> GKDNFDAPESKLVGRVTYQGQALNLRGTG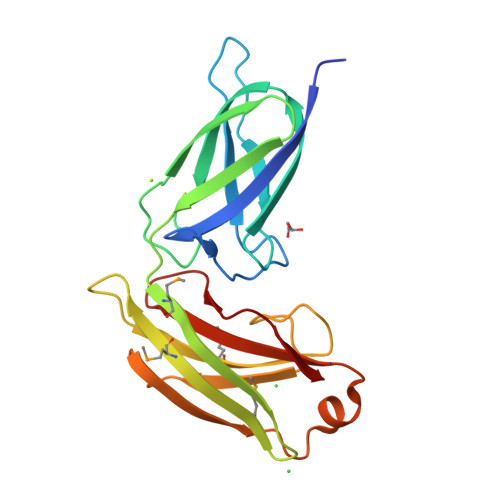EAVQLQLYQDGYEKNDPISVFVGQDGTFSALLFDGEYRLTTRDGNGPWVNNHESVTVNLKGHTEVNLEVTPYFMISNEQLSVTGSAMNASFMINRIVPDAKISRVMLLLSKTQFADDVNNLYRQDFSDVVPGSVNLSADISGNTEIVKAKALYARVGVLANGADQAIYSPVVRLK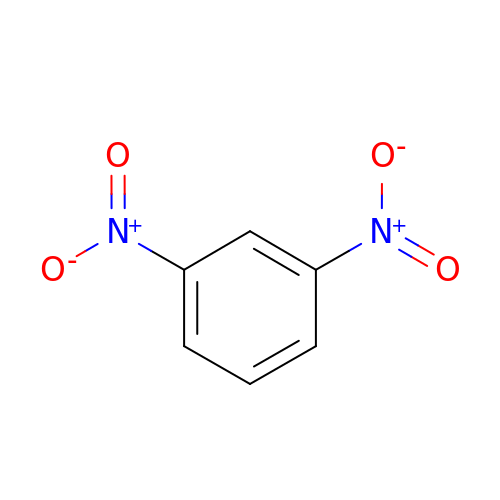DINITROPHENYLENE | C6 H4 N2 O4 | WDCYWAQPCXBPJA-UHFFFAOYSA-N>SNAIRPTIGQQMETGDQRFGDLVFRQLAPNVWQHTSYLDVPGFGAVASNGLIVRDGGRVLVVDTAWTDDQTAQILNWIKQEINLPVALAVVTHAHQDKMGGMDALHAAGIATYANALSNQLAPQEGMVAAQHSLTFAANGWVEPATAPNFGPLKVFYPGPGHTSDNITVGIDGTDIAFGGCLIK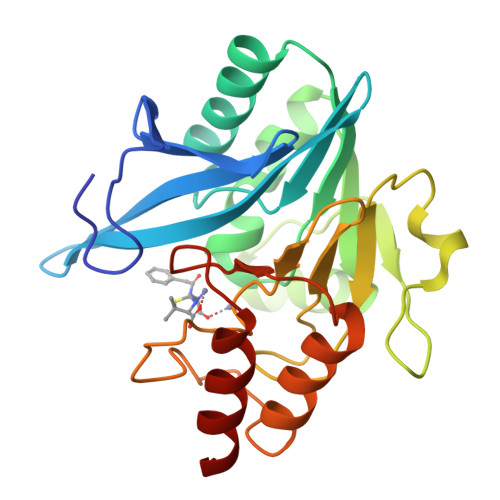DSKAKSLGNLGDADTEHYAASARAFGAAFPKASMIVMSHSAPDSRAAITHTARMADKLR[2x]Here, we report the first structure of glycerol kinase from the thermophilic filamentous fungus Chaetomium thermophilum (CtGK). Glycerol kinase (EC 2.7.1.30) catalyzes the transfer of phosphate moiety from ATP to glycerol to form glycerol 3-phosphate (G3P). Overall, the CtGK polypeptide chain can be divided into two distinct domains classified by Pfam as FGGY_N (residues 65–325) and FGGY_C (residues 331–583) connected by a flexible region. A similar case is found in CtGK, which forms extended dimers via the interaction between the C-terminal domains with a prominent contribution from hydrophobic residues (Phe422, Gly436, Phe389, Leu394, Thr437, Phe439, Gly440, Ile441, Thr437, Thr445, Leu438, Ile450, Trp580).

Subsequently, by replacing the cryoprotectant solution with 20–25% glycerol, we were able to solve the enzyme-substrate complex with a clear electron density that could be attributed to the bound glycerol moiety. In total, three different crystal structures were obtained in the presence of glycerol, constituting 13 polypeptide chains. Generally, the same extent of the chain could be modeled as in the apo structures, i.e., for residues 65–583 with an approximate 9aa gap between H18 and B18. The substrate is bound in an evolutionarily conserved cleft within the N-terminal domain that opens towards the C-terminal domain. The glycerol molecule is coordinated by polar interactions with side chains of Glu149, Arg 148, Asp317, Gln318, and additionally with Arg148 main-chain amide. The carbon chain of glycerol packs against hydrophobic Trp168 and Phe342. A similar mode of binding was described previously for P. falciparum GK, where Phe271 and Tyr135 undergo shift upon substrate or cofactor binding. However, the movement of equivalent residues (Phe342 and Tyr200) was not observed in either of the presented CtGK complexes. Of note, we solved and refined five CtGK structures, and each of them belongs to a different space group, despite crystals having grown in the same buffer condition. We observed that in the absence of nucleotide, CtGK adopts open conformation, which upon nucleotide binding closes up.

>[4x]GSFVGSIDQGTTSSRFLIFNGEGNPVASHQIEFENLYPKSGWHEQDPYELLNSVQQCIDGAMHKFASLGYSKENIRAIGITNQRETTVVWDSVTGEPLHNAIVWPDTRTSALVRELKARQSADSLLELCGLPLSTYPSSVKLLWLIQNVDAVKQAYEEGRLAFGTVDSWLIYKLNGGAQAERPIHVTDSTNASRTMFMNLRTLQYDDKLLGFFGIDRNKIKLPKIVPSSDPEAFGKVATGALAGVPIAGCLGDQSSALVGQCGFSPGQAKNTYGTGCFLLYNVGTEPVISKYGLLATVAYDFGRGRKPVYALEGSIAVAGAGITFLMNNLGFAPKPSEINALAESVLDNGGVVFVTAFSGLFAPYWIDDAKGTLFGITQHTTKGHIARATLEATCYQTRAILDAMEKDSGHKLESLAVDGGLSASDLCMQTQADISGIPVDRPRMRETTALGAAIAAGLATGVWRELDHVKESIAGGANGNGKKNAREVFYPKMDRKKAERLFRKWEQAVEMSRGWVREQEEEDGE2-[5-(3-chloro-4-{[(1R)-1-(2-fluorophenyl)ethyl]amino}quinolin-6-yl)pyrimidin-2-yl]propan-2-ol 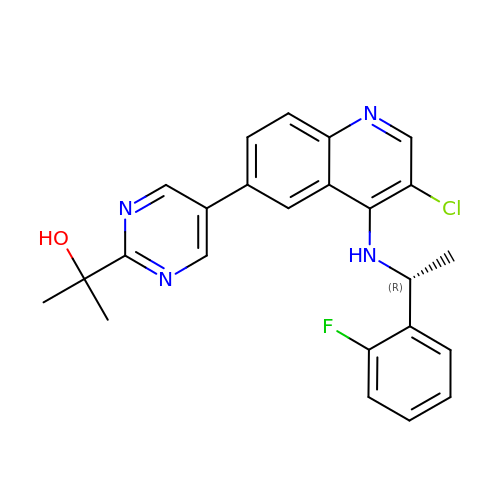| C24 H22 Cl F N4 O | TZXWJHVVESOPPE-CQSZACIVSA-N> SNAPLGQT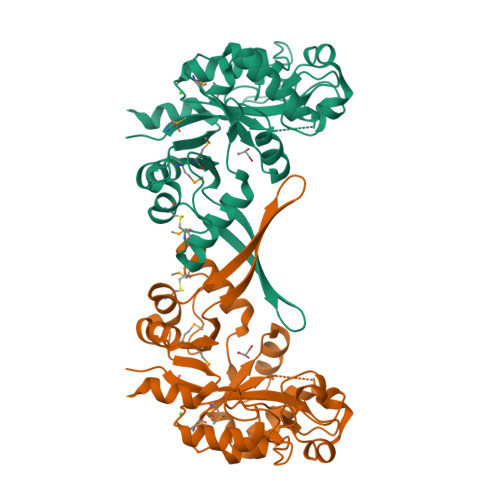DDPMIVAHRAGTRDFPENTVLAITNAVAAGVDGMWLTVQVSSDGVPVLYRPSDLATLTDGAGPVNSKTVQQLQQLNAGWNFTTPGVEGHPYRQRATPIPTLEQAIGATPPDMTLFLDLKQTPPQPLVSAVAQVLTRTGAAGRSIVYSTNADITAAASRQEGLQVAESRDVTRQRLFNMALNHHCDPQPDPGKWAGFELHRDVTVTEEFTLGSGISAVNAELWDEASVDCFRSQSGMKVMGFAVKTVDDYRLAHKIGLDAVLVDSPLAAQQWRH> 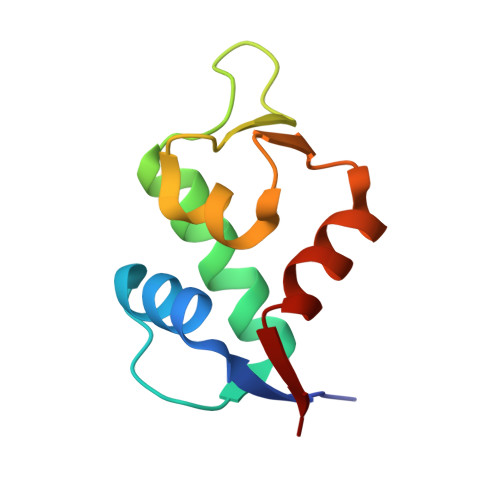MQETLVRPKPLLLKLLKSVGAQKDTYTMKEVLFYLGQYIMTKRLYDEKQQHIVYCSNDLLGDLFGVPSFSVKEHRKIYTMIYRNLVVV>[2x]MIITVASFKGGVGKTTTAVHLSAYLALQGETLLIDGDPNRSATGWGKRGSLPFKVVDERQAAKYAPKYQNIVIDTQARPEDEDLEAL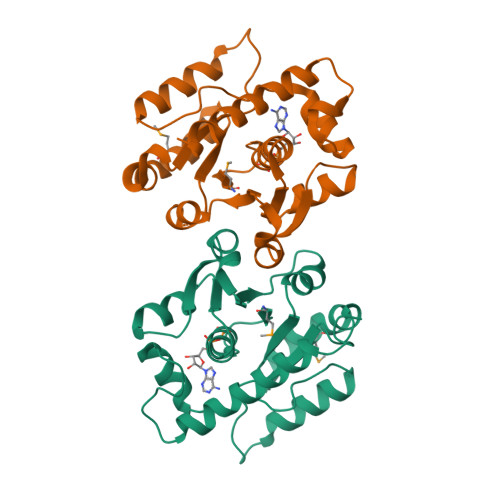ADGCDLLVIPSTPDALALDALMLTIETLQKLGNNRFRILLTIIPPYPSKDGDEARQLLTTAGLPLFKRGIKRYSAFQKASLNGVVVSEVSDSKAGIAWSDYKATGKEIVEEILTLEHHHHHH> IINGEDCSPHSQPWQAALVMENELFCSGVLVHPQWVLSAAHCFQNSYTIGLGLHSLEA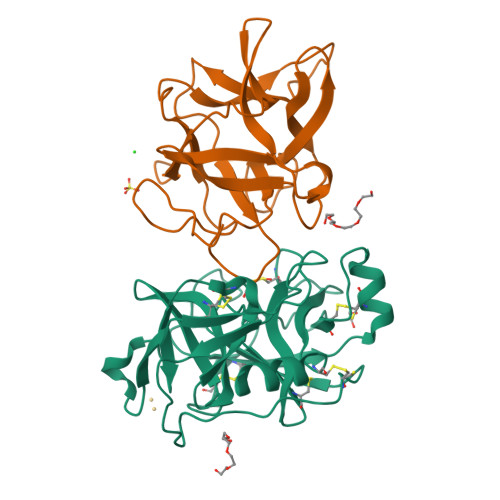DQEPGSQMVEASLSVRHPEYNRPLLANDLMLIKLDESVSESDTIRSISIASQCPTAGNSCLVSGWGLLANGRMPTVLQCVNVSVVSEEVCSKLYDPLYHPSMFCAGGGQDQKDSCNGDSGGPLICNGYLQGLVSFGKAPCGQVGVPGVYTNLCKFTEWIEKTVQA;> GSSVVVDTNGQPVSNGADAYYLVPVSHGHAGLALAKIGNEAEPRAVVLDPHHRPGLPVRFESPLMINIIKESYFLNIKFGPSSSDSGVWDVIQQDPIGLAVKVTDTKSLLGPFKVEKEGEGYKIVYYPERGQTGLDIGLVHRNDKYYLAVKDGEPCVFKIRKATDE> MGGSEVGTVPVTWRLGVDVGERSIGLAAVSYEEDKPKEILAAVSWIHDGGVGDERSGASRLALRGMARRARRLRRFRRARLRDLDMLLSELGWTPLPDKNVSPVDAWLARKRLAEEYVVDETERRRLLGYAVSHMARHRGWRNPWTTIKDLKNLPQPSDSWERTRESLEARYSVSLEPGTVGQWAGYLLQRAPGIRLNPTQQSAGRRAELSNATAFETRLRQEDVLWELRCIADVQGLPEDVVSNVIDAVFCQKRPSVPAERIGRDPLDPSQLRASRACLEFQEYRIVAAVANLRIRDGSGSRPLSLEERNAVIEALLAQTERSLTWSDIALEILKLPNESDLTSVPEEDGPSSLAYSQFAPFDETSARIAEFIAKNRRKIPTFAQWWQEQDRTSRSDLVAALADNSIAGEEEQELLVHLPDAELEALEGLALPSGRVAYSRLTLSGLTRVMRDDGVDVHNARKTCFGVDDNWRPPLPALHEATGHPVVDRNLAILRKFLSSATMRWGPPQSIVVELGGGSAGGYAAVALRDRLLSYGEKNGVAQVAVFRGGVTAEARRWLDISIERLFSRVAIFAQSTSTKRLDRRHHAVDAVVLTTLTPGVAKTLADARSRRVSAEFWRRPSDVNRHSTEEPQSPAYRQWKESCSGLGDLLISTAARDSIAVAAPLRLRPTGALHEETLRAFSEHTVGAAWKGAELRRIVEPEVYAAFLALTDPGGRFLKVSPSEDVLPADENRHIVLSDRVLGPRDRVKLFPDDRGSIRVRGGAAYIASFHHARVFRWGSSHSPSFALLRVSLADLAVAGLLRDGVDVFTAELPPWTPAWRYASIALVKAVESGDAKQVGWLVPGDELDFGPEGVTTAAGDLSMFLKYFPERHWVVTGFEDDKRINLKPAFLSAEQAEVLRTERSDRPDTLTEAGEILAQFFPRCWRATVAKVLCHPGLTVIRRTALGQPRWRRGHLPYSWRPWSADPWSTAEL

Here we further characterized the PAM recognized by AceCas9 and report crystal structures of AceCas9 without its HNH domain (AceCas9–ΔHNH) bound with a guide RNA and DNA targets. Similar to other Cas9, AceCas9 contains the conserved RuvC domain that is connected by the arginine-rich bridge helix (BH) to the nucleic acid recognition domain (REC) and the PAM-interacting domain (PID). Unlike other Cas9, AceCas9 functions at an elevated temperature, interacts with its specific RNA partner, and recognizes the unique 5′-NNNCC-3′ PAM. We show that AceCas9 contacts the 5′-NNNCC-3′ PAM by forming a network of hydrogen bonds with both the cytosine and guanine bases.

A truncated but active guide RNA, sgRNA94, a target strand (TS) DNA comprised of the 20-nt complementary and a 10-nt PAM region, and a nontarget strand (NTS) DNA that base pairs with the PAM region of the TS allowed cocrystallization with AceCas9–ΔHNH. The structure of the ternary complex was solved by a combination of molecular replacement and single-wavelength anomalous diffraction methods and refined at 2.9 Å to crystallographic residual factors of 0.22/0.26 (R/Rfree) (“Methods”). In the final model, we were able to place 949 of the total 988 protein residues, 91 of the 94 sgRNA94 nucleotides including the first triphosphate nucleotide (G1), and all of the DNA nucleotides. The ternary complex crystal structure reveals specific interaction of the 5′-NNNCC-3′ PAM with AceCas9 residues in its PI subdomain. Specifically, the carboxylate group of Glu1044 contacts the exocyclic amino of C4* on NTS and the guanidinium groups of Arg1088 and Arg1091 contact the exocyclic oxygen of G(-4) and G(-5) on TS, respectively. In addition, Arg1091 establishes a salt bridge with Glu1044 to further enhance the Glu1044-C4*-Arg1091-G(-5) network of interactions. This PAM-interaction network explains the specificity of AceCas9 for the 5′-NNNCC-3′ PAM and its methylation state, although it does not explain why 5′-NNNAC-3′ is a weak PAM. Mutation of Glu1044 or Arg1091 significantly reduced the DNA cleavage activity while that of Arg1088 moderately reduced the activity. AceCas9 residues directly contact C4* of the nontarget strand and G(-5)-G(-4) of the target strand. Accordingly, methylation of C4* but not C5* abolishes the DNA cleavage activity of AceCas9.>SNATKKSAAEASKKPRQKRTATKAYNVTQAFGRRGPEQTQGNFGDQELIRQGTDYKHWPQIAQFAPSASAFFGMSRIGMEVTPSGTWLTYTGAIKLDDKDPN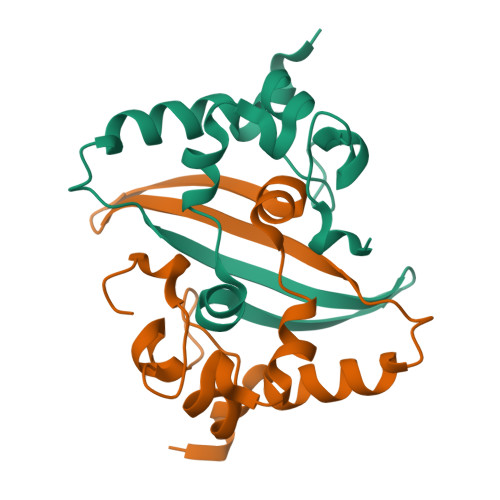FKDQVILLNKHIDAYKTFP[4x]> NIPFTNNLLFSGQVLYGDGRLTAKSHQLVMQGDCNLVLYGGKYGWQSNTHGNGEHCFLRLNHKGEL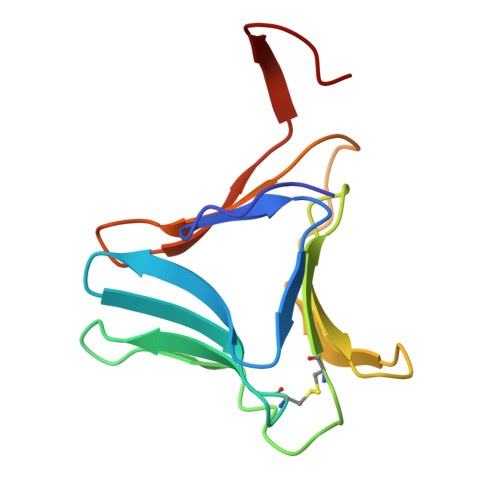IIKDDDFKTIWSSSSSSKHGDYVLILRDDGFAVIYGPAIWETSPQA>MASTVLNVPIAQPENGSSDKIPKWSARAIKSLAMGELEARKLKYPSTGTEAILMGILVEGTSTVAKFLRGNGVTLFKVRDETLSLLGKSDMYFFSPEHPPLTEPAQKAIAWAIDEKNKSDVDGELTTAYLLLGVW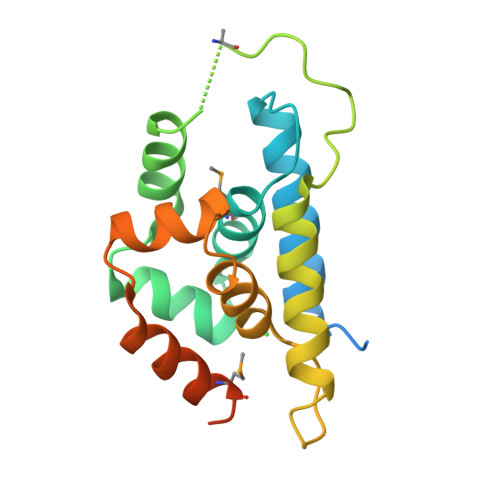SQKDSAGRQILEKLGFNEDKAKEVEKSMNEDVDLSFKKQGQLEHHHHHH[2x]4-cyano-N-{3-[1-(cyclohexanecarbonyl)piperidin-4-yl]-1-methyl-1H-indol-5-yl}pyridine-2-carboxamide 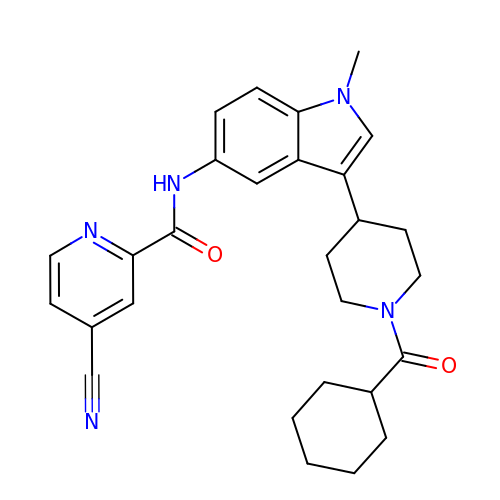| C28 H31 N5 O2 | LRJCIDHTWFKTMZ-UHFFFAOYSA-N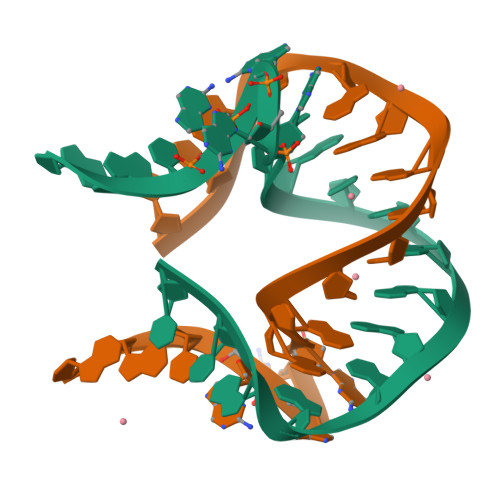>GGCGGGGAACCGGGGAGCC[4x]SULFANYLACETIC ACID | C2 H4 O2 S | 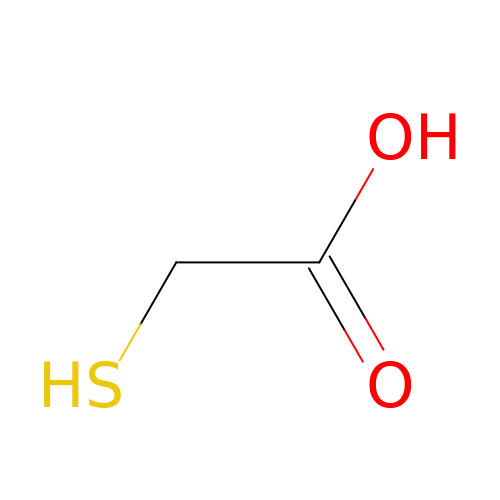CWERGRDVMFNCDR-UHFFFAOYSA-N>MGSSHHHHHHSSSAALEVLFQGPAPEDLLERLLGEMELELIELRRALAQTIATFKSTERQRDAQQLIAQRWYEKAQAALDRGNEQLAREALGQRQSYQSHTEALGKSLGEQRALVEQVRGQLQKLERKYLELKSQKNLYLARLKSAIAAQKIEEIAGNLDNASASSLFERIETKILELEAERELLNPPPSPLDKKFEQWEEQQAVEATLAAMKARRSLPPPSS[60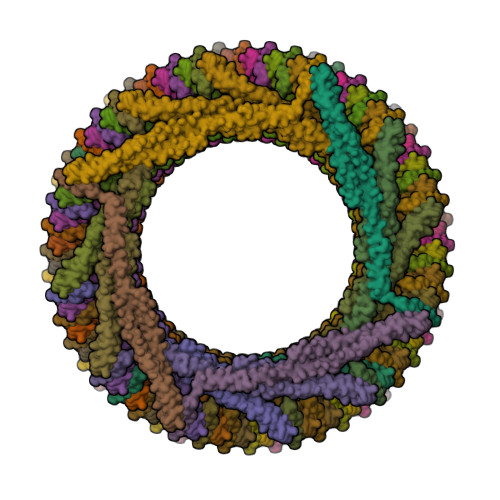x]>GPLGSEWSSSQPATGEKKECWSWESYLEEQKAITAPVSLFQDSQAVTHNKNGFKLGMKLEGIDPQHPSMYFILTVAEVCGYRLRLHFDGYSECHDFWVNANSPDIHPAGWFEKTGHKLQPPKGYKEEEFSWSQYLRSTRAQAAPKHLFVSQSHSPPPLGFQVGMKLEAVDRMNPSLVCVASVTDVVDSRFLVHFDNWDDTYDYWCDPSSPYIHPVGWCQKQGKPLTPPQDYPDPDNFCWEKYLEETGASAVPTWAFKVRPPHSFLVNMKLEAVDRRNPALIRVASVEDVEDHRIKIHFDGWSHGYDFWIDADHPDIHPA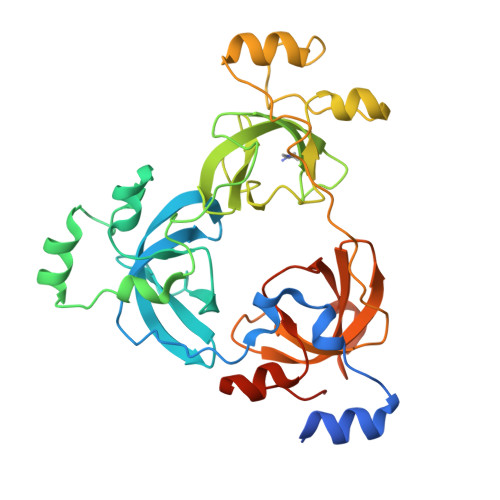GWCSKTGHPLQPPLGPREPSSASPGG[3x];>TSRHKKLMFK[2x]> HMCNKNNTFEKNLDISHKPEPLILFNKDNNIWNSKYFRIPNIQLLNDGTILTFSDIRYNGPDDHAYIDIASARSTDFGKTWSYDIAMKNNRIDSTYSRVMDSTTVITNTGRIILIAGSWNTNGNWAMTTSTRRSDWSVQMIYSDDNGLTWSNKIDLTKDSSKVKNQPSNTIGWLGGVGSGIVMDDGTIVMPAQISLRENNENNYYSLIIYSKDNGETWTMGNKVPNSNTSENMVIELDGALIMSTRYDYSGYRAAYISHDLGSTWEIYEPLNGKVLTGKGSGCQGSFIKATTSNGHRIGLISAPKNTKGEYIRDNIAVYMIDFDDLSKRVQEICIPYPKDGNKLGGGYSCLSFKNSHLSIVYEANGNIEYQDLTPYYSLINKQ

The genomes of most C. perfringens strains contain three separate genes encoding highly conserved GH33 CAZymes targeting sialic acid glycosidic linkages: the nonsecreted 43 kDa NanH, and the two secreted 77 kDa NanI and 129 kDa NanJ. Here, we present the structural and biochemical characterization of the GH33 catalytic domains of the three sialidases of C. perfringens and probe their substrate specificity. The catalytically active domains, which we refer to as NanHGH33, NanJGH33, and NanIGH33, displayed differential activity on various naturally occurring forms of sialic acid. We report the X-ray crystal structures of these domains in complex with relevant sialic acid variants revealing the molecular basis of how each catalytic domain accommodates different sialic acids.

NanH consists solely of the catalytic GH33 domain. The structures of NanHGH33 and NanJGH33 display the characteristic 6-bladed β-propeller fold seen in exo-acting sialidase GH33 domains. The inserted domain is not present in NanHGH33 and the RMSD of NanHGH33 with the other two structures is 1.7 Å. NanHGH33, however, has a considerably different organization in the active site region that interacts with the glycerol moiety, suggesting this may contribute to the ability of this enzyme to recognize additional acetylated variants of sialic acid. The most notable difference in NanH is in the loop structures surrounding the active site. In NanHGH33 loops on 3-blades forming the rim of one side of the cavity are extended, thus deepening the active site. The center blade of the three has a solvent exposed tyrosine residue, Y310, that projects into the active site. In contrast, NanH is predicted to be localized to the cytoplasm of the bacterium (i.e. it lacks any obvious export signals), suggesting it does not interact directly with the host. The biological role of NanH is more likely in processing glycans that are imported with their terminal sialic acids intact.>GQDMVSPPPPIADEPLTVNTGIYLIECYSLDDKAETFK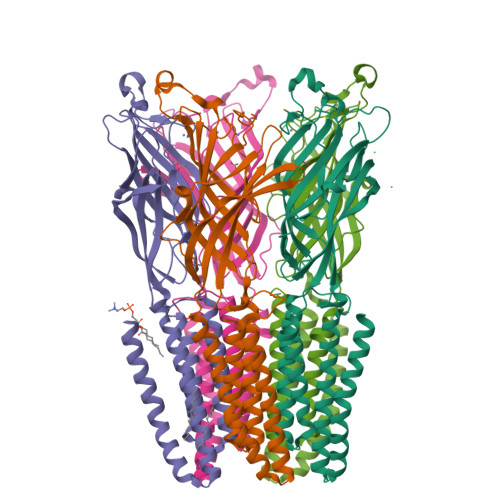VNAFLSLSWKDRRLAFDPVRSGVRVKTYEPEAIWIPEIRFVNVENARDANVVDISVSPDGTVQYLERFSARVLSPLDFRRYPFDSQTLHIYLIVRSVDTRNIVLAVDLEKVGKNDDVFLTGWDIESFTAVVKPANFALEDRLESKLDYQLRISRQYFSYIPNIILPMLFILFISWTAFWSTSYEANVTLVVSTLIAHIAFNILVETNLPKTPYMTYTGAIIFMIYLFYFVAVIEVTVQHYLKVESQPARAASITRASRIAFPVVFLLANIILAFLFFGF[5x]>[16x]APAADAAQAHDPLSVQTGSDIPASVHMPTDQQRDYIKREVMVPMRDGVKLYTVIVIPKNARNAPILLTRTPYN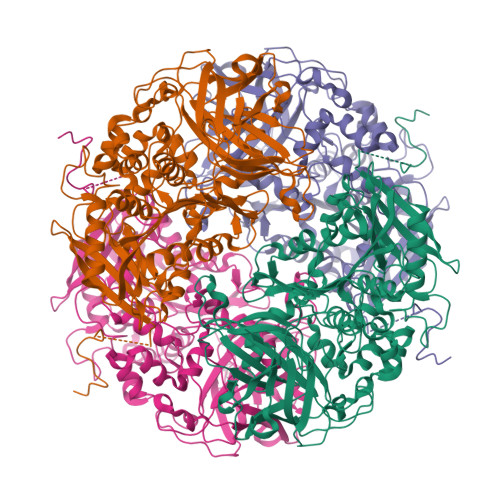AKGRANRVPNALTMREVLPQGDDVFVEGGYIRVFQDIRGKYGSQGDYVMTRPPHGPLNPTKTDETTDAWDTVDWLVHNVPESNGRVGMTGSSYEGFTVVMALLDPHPALKVAAPESPMVDGWMGDDWFHYGAFRQGAFDYFVSQMTARGGGNDIPRRDADDYTNFLKAGSAGSFATQAGLDQYPFWQRMHAHPAYDAFWQGQALDKILAQRKPTVPMLWEQGLWDQEDMWGAIHAWQALKDADVKAPNTLVMGPWRHSGVNYNGSTLGPLEFEGDTAHQYRRDVFRPFFDEYLKPGSASVHLPDAIIYNTGDQKWDYYRSWPSVCESNCTGGLTPLYLADGHGLSFTHPAADGADSYVSDPAHPVPFISRPFAFAQSSRWKPWLVQDQREAESRPDVVTYETEVLDEPVRVSGVPVADLFAATSGTDSDWVVKLIDVQPAMTPDDPKMGGYELPVSMDIFRGRYRKDFAKPEALQPDATLHYHFTLPAVNHVFAKGHRIMVQIQSSWFPLYDRNPQKFVPNIFDAKPADYTVATQSIHHGGKEATSILLPVVKQKLGPEQKLISEEDLNSAVDHHHHHH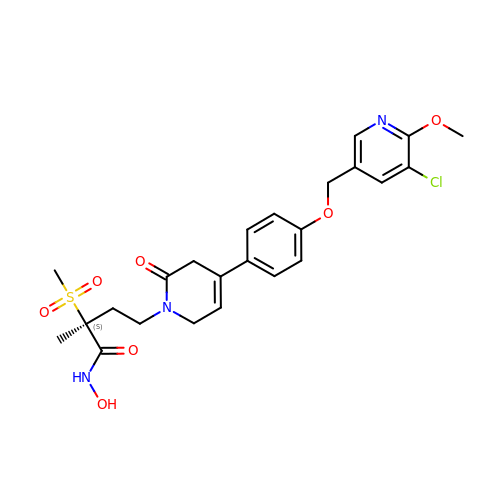(2S)-4-[4-{4-[(5-chloro-6-methoxypyridin-3-yl)methoxy]phenyl}-2-oxo-3,6-dihydropyridin-1(2H)-yl]-N-hydroxy-2-methyl-2-(methylsulfonyl)butanamide | C24 H28 Cl N3 O7 S | CDFIGPHKVBKXMP-DEOSSOPVSA-N> MEKVYQAGTHEGMIDFINMEDLELAATQVIPSGGYGYISSGAGDLFTYRENQKAFNHQLVIPHVLKDVELPDTTTYFSDETLAAPIIMAPVAAHGLAHEQAEKASAKGVSEFGTIYTASSYASCTLEEIRAAGGPEAPQWFQFYMSKDDGINLDILEMAKRNGAKAVVLTADATVGGNRETDRRNGFTFPLPMPIVQAYQSGVGQTMDAVYKSSKQ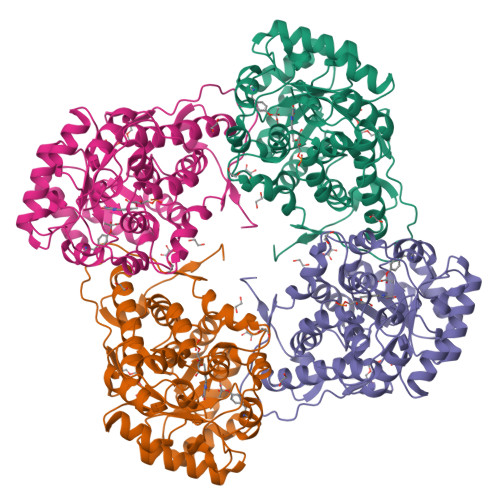KLSPKDIEFITTHSELPVYVKGVQSEDDVYRSLDAGAQGIWVSNHGGRQLDGGPASFDSLRYVAEAVDKRVPIVFDSGVRRGQHIFKAIASGADLVAIGRPAIYGLSLGGSTGIKQVFDFFKTELEMVMQLAGTQTVEDIKNAKLRENRFMC>[2x]MGSPFLRGTVEKEVTKVKQSIEDELIRSDSQLMNFPQLPSNGIPQDDVIEELNKLNDLIPHTQWKEGKVSGAVYHGGDDLIHLQTIAYEKYCVANQLHPDVFPAVRKME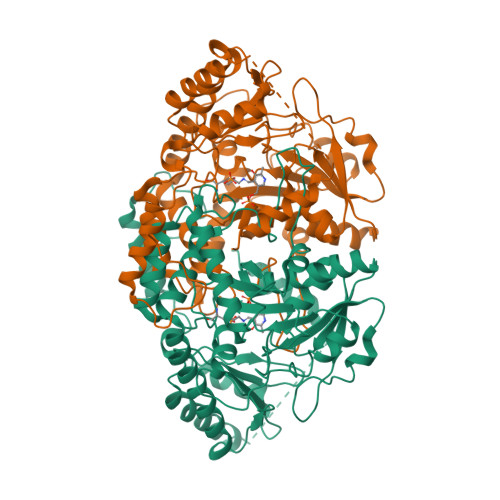SEVVSMVLRMFNAPSDTGCGTTTSGGTESLLLACLSAKMYALHHRGITEPEIIAPVTAHAGFDKAAYYFGMKLRHVELDPTTYQVDLGKVKKFINKNTVLLVGSAPNFPHGIADDIEGLGKIAQKYKLPLHVDSCLGSFIVSFMEKAGYKNLPLLDFRVPGVTSISCDTHKYGFAPKGSSVIMYRNSDLRMHQYYVNPAWTGGLYGSPTLAGSRPGAIVVGCWATMVNMGENGYIESCQEIVGAAMKFKKYIQENIPDLDIMGNPRYSVISFSSKTLNIHELSDRLSKKGWHFNALQKPVALHMAFTRLSAHVVDEICDILRTTVQELKSESNSKPSPDGTSALYGVAGSVKTAGVADKLIVGFLDALYKLGPGEDTATKLEHHHHHH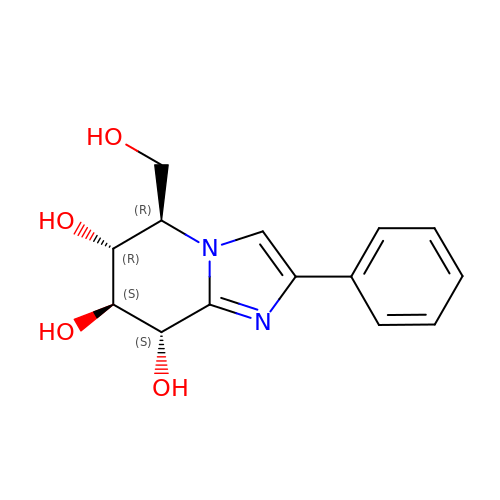(5R,6R,7S,8S)-5-(HYDROXYMETHYL)-2-PHENYL-5,6,7,8-TETRAHYDROIMIDAZO[1,2-A]PYRIDINE-6,7,8-TRIOL | C14 H16 N2 O4 | DLVNFMROYKHANV-FVCCEPFGSA-N>DTGCAVSWSGKELKCGSGIFVIDNVHTWTEQYK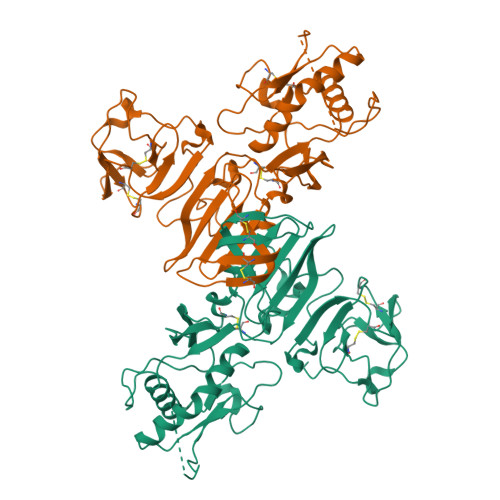FQPESPARLASAILNAHEDGVCGIRSTTRLENIMWKQITNELNYVLWEGGHDLTVVAGDVKGVLSKGKRALAPPVNDLKYSWKTWGKAKIFTPEAKNSTFLIDGPDTSECPNERRAWNFLEVEDYGFGMFTTNIWMKFREGSSEVCDHRLMSAAIKDQKAVHADMGYWIESSKNQTWQIEKASLIEVKTCLWPKTHTLWSNGVLESQMLIPKAYAGPFSQHNYRQGYATQTVGPWHLGKLEIDFGECPGTTVTIQEDCDHRGPSLRTTTASGKLVTQWCCRSCTMPPLRFLGEDGCWYGMEIRPLSEKEENMVKSQVSAHHHHHH[2x]Formation of this complex catalytic core in the large subunit of [NiFe]-hydrogenase requires accessory proteins encoded by genes designated hypA to hypF in the hyp operon. After delivery of the Fe(CN)2CO complex to the large subunit precursor, nickel is transferred to the precursor with aid of protein HypA and HypB. HypB belongs to the SIMIBI class GTPase with slow intrinsic GTP hydrolysis activity. Many GTPases, including HypB, undergo GTP-induced dimerization and in a recent review, Gasper et al. categorized them as “G proteins activated by nucleotide-dependent dimerization”.

The only structure of HypB available was the MjHypB in complex with GTPγ-S. To better understand the structural mechanism of GTP-dependent dimerization, we have determined the crystal structure of HypB from A. fulgidus (AfHypB) in apo form to 2.3 Å. Each asymmetric unit contains 2 monomers of AfHypB. AfHypB belongs to the SIMIBI class of GTPase and adopts an α/β fold with a seven-stranded beta-sheet sandwiched by 11 α-helices. Electron density of residues 67–82, corresponding to the switch I region, of chain B are missing, indicating that these residues are not ordered. In contrast, we found that symmetry-related AfHypB molecules may restrict the mobility of switch I of chain A, and hence, these residues are well defined in chain A. Besides, the side-chain sulphur atoms of two cysteine residues, Cys-92 and Cys-122, which are part of the CHxnC motif, of apo-AfHypB structure are in 2 Å distance, suggesting the formation of a disulphide bridge between these two residues. In AfHypB, the conserved Asp residue in the NKxD motif is replaced by an Ala residue. We have superimposed the structures of AfHypB and MjHypB, and found that there is a nearby Asp-194 on the G5 loop, away from the G4 motif, that can form a hydrogen bond to the N1 atom of the guanine nucleotide. Modeling suggests that the binding pocket in apo-HypB can accommodate a GDP but is too small to accommodate a GTP as the γ-phosphate will clash with an invariant aspartate residue (Asp-66 in AfHypB) on the G2 loop. First, in the apo-form, Asp-66 on the G2 loop is anchored to Gly-118 and Lys-43 by two hydrogen bonds, which are broken in the GTPγS-bound MjHypB.

>[2x]MHEYELNQDLLAENKRLAEKNREALRESGTVAVNIMGAIGSGKTLLIERTIERIGNEVKIGAMLGDVVSKADYERVRRFGIKAEAISTGKECHLDAHMIYHRLKKFSDCDLLLIENVGNLICPVDFDLGENYRVVMVSVTEGDDVVEKHPEIFRVADLIVINKVALAEAVGADVEKMKADAKLINPRAKIIEMDLKTGKGFEEWIDFLRGILNVHSDSGQN>GCCCGGAUAGCUCAGUCGGUAGAGCAGCGGGCACUAUGGGCGCAGUGUCAAUGG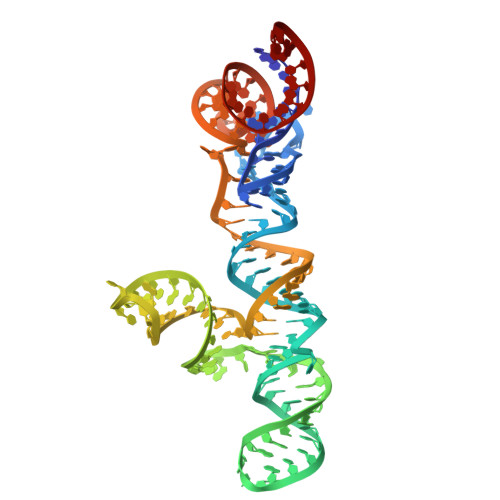ACGCUGACGGUACAGGCCAGACAAUUAUUGUCUGGUAUAGUGCCCGCGGGUCCAGGGUUCAAGUCCCUGUUCGGGCGCCA[2x]>GSHMSEQLTDQVLVERVQKGDQKAFNLLVVRYQHKVASLVSRYVPSGDVPDVVQEAFIKAYRALDSFRGDSAFYTWLYRIAVNTAK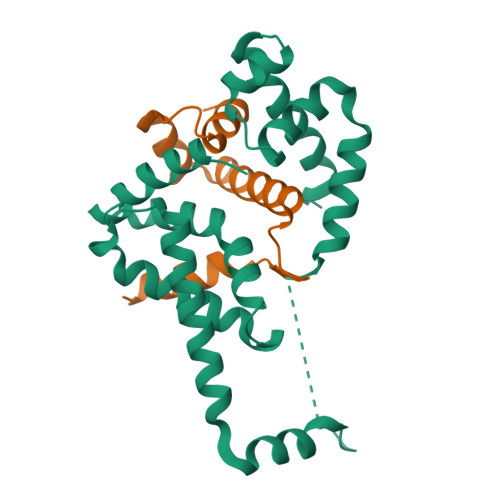NYLVAQGRRPPSSDVDAIEAENFESGGALKEISNPENLMLSEELRQIVFRTIESLPEDLRMAITLRELDGLSYEEIAAIMDCPVGTVRSRIFRAREAIDNKVQPLIRR[2x];>MQKEQLSALMDGETLDSELLNELAHNPEMQKTWESYHLIRDSMRGDTPEVLHFDISSRVMAAIEEEPVRQPATLIPEAQPAPHQWQKMPF[2x]>[3x]PMFIVNTNVPRASVPD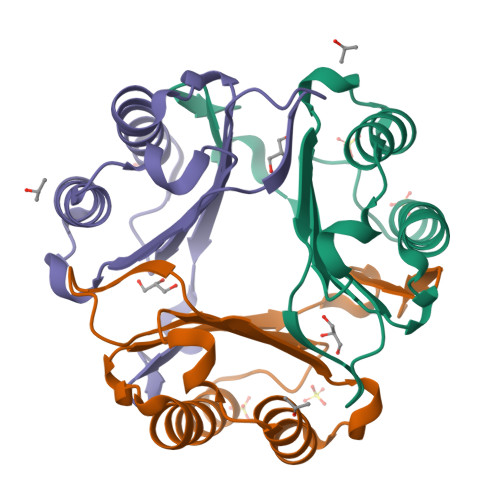GFLSELTQQLAQATGKPPQYIAVHVVPDQLMAFGGSSEPCALCSLHSIGKIGGAQNRSYSKLLCGLLAERLRISPDRVYINYYDMAAANVGWNNSTFA> GGIVNVSERHSCPLGFGHYSVVDVCIFETVVIVLLTFLIIAGNLTVIFVFHCAPLLHHYTTSYFIQTMAYADLFVGVSCLVPTLSLLHYSTGVHESLTCQVFGYIISVLKSVSMWCLACISVDRYLAITKPLSYNQLVTPCRLRICIILIWIYSCLIFLPSFFG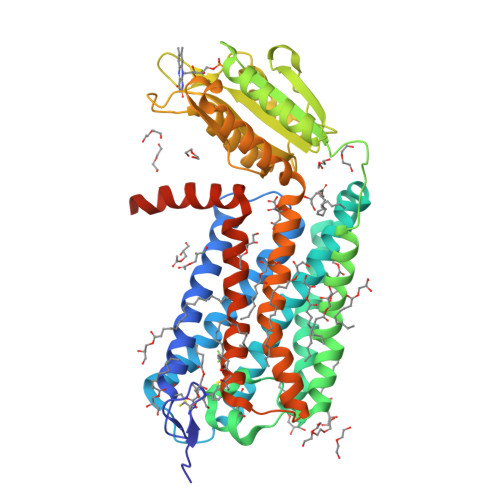WGKPGYHGDIFEWCATSWLTSAYFTGFIVCLLYAPAAFVVCFTYFHIFKICRQHTKEAKALIVYGSTTGNTEYTAETIARELADAGYEVDSRDAASVEAGGLFEGFDLVLLGCSTWGDDSIELQDDFIPLFDSLEETGAQGRKVACFGCGDSSWEYFCGAVDAIEEKLKNLGAEIVQDGLRIDGDPRAARDDIVGWAHDVRGAIRRYLMVLFRITSVFYMLQLPYIIYFLLESSRVLDNPTLSFLTTWLAISNSFCNPVIYALSDSTFRLGLRRLSETMCTSCMEFLEVLFQGPHHHHHHHHHH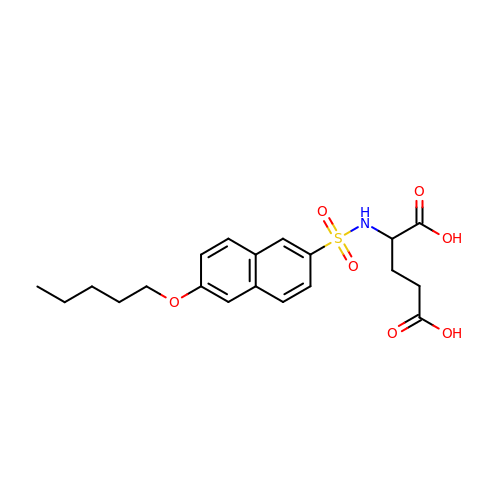N-{[6-(PENTYLOXY)NAPHTHALEN-2-YL]SULFONYL}-D-GLUTAMIC ACID | C20 H25 N O7 S | LIGACKDHLKEZFH-GOSISDBHSA-N>MAEKRTGLAEDGAKSVYERLKNDRAPYETRAQNCAQYTIPSLFPKDSDNASTDYQTPWQAVGARGLNNLASKLMLALFPMQTWMRLTISEYEAKQLLSDPDGLAKVDEGLSMVERIIMNYIESNSYRVTLFEALKQLVVAGNVLLYLPEPEGSNYNPMKLYRLSSYVVQRDAFGNVLQMVTRDQIAFGALPEDIRKAVEGQGGEKKADETIDVYTHIYLDEDSGEYLRYEEVEGMEVQGSDGTYPKEACPYIPIRMVRLDGESYGRSYIEEYLGDLRSLENLQ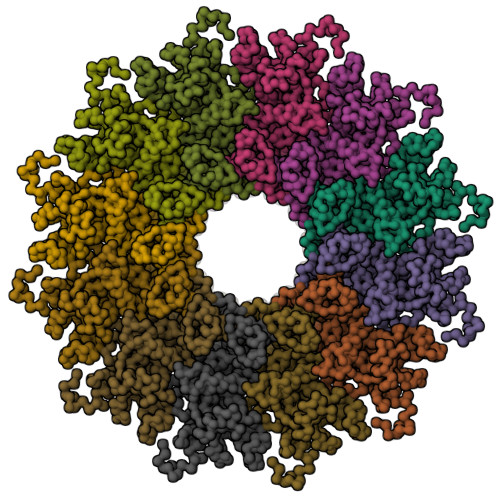EAIVKMSMISSKVIGLVNPAGITQPRRLTKAQTGDFVTGRPEDISFLQLEKQADFTVAKAVSDAIEARLSFAFMLNSAVQRTGERVTAEEIRYVASELEDTLGGVYSILSQELQLPLVRVLLKQLQATQQIPELPKEAVEPTISTGLEAIGRGQDLDKLERCVTAWAALAPMRDDPDINLAMIKLRIANAIGIDTSGILLTEEQKQQKMAQQSM[12x]>[2x]MKNVGFIGWRGMVGSVLMDRMSQENDFENLNPVFFTTSQAGQKAPVFGGKDAGDLKSAFDIEELKKLDIIVTCQGGDYTNEVYP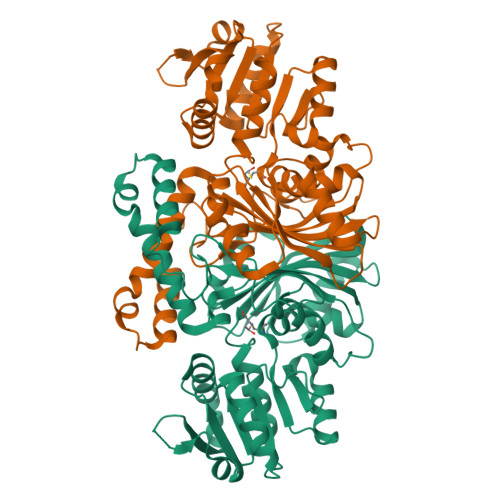KLKATGWDGYWVDAASALRMKDDAIIVLDPVNQHVISEGLKKGIKTFVGGNCTVSLMLMAIGGLFEKDLVEWISVATYQAASGAGAKNMRELLSQMGLLEQAVSSELKDPASSILDIERKVTAKMRADNFPTDNFGAALGGSLIPWIDKLLPETGQTKEEWKGYAETNKILGLSDNPIPVDGLCVRIGALRCHSQAFTIKLKKDLPLEEIEQIIASHNEWVKVIPNDKEITLRELTPAKVTGTLSVPVGRLRKLAMGPEYLAAFTVGDQLLWGAAEPVRRILKQLVA> APARGTLLTSNFLTSY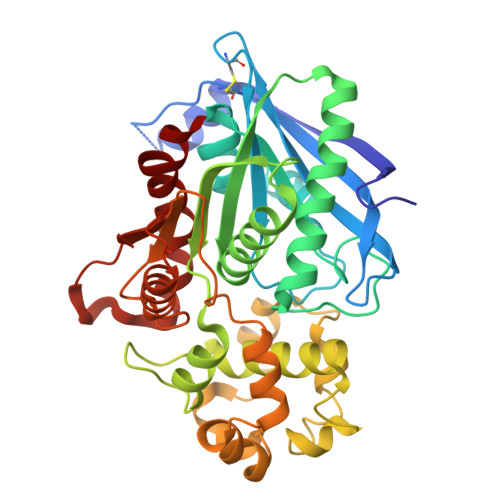TRDAISAMLASGSQPASGSQPEQAKCNVRVAEFTYATIGVEGEPATASGVLLIPGGERCSGPYPLLGWGHPTEALRAQEQAKEIRDAKGDDPLVTRLASQGYVVVGSDYLGLGKSNYAYHPYLHSASEASATIDAMRAARSVLQHLKTPLSGKVMLSGYSQGGHTAMATQREIEAHLSKEFHLVASAPISGPYALEQTFLDSWSGSNAVGENTFFILLGSYAIVAMQHTYKNIYLEPGQVFQDPWAAKVEPLFPGKQSLTDMFLNDTLPSIDKVKSYFQPGFYSDFPSNPANPFRQDLARNNLLEWAPQTPTLLCGSSNDATVPLKNAQTAIASFQQRGSNQVALVDTGTGNASDNSAFAHMLTKESCIVVVRDQLLDKQR>[4x]MSLTIGVIGKSVHPYWSQVEQGVKAAGKALGVDTKFFVPQKEDINAQLQMLESFIAEGVNGIAIA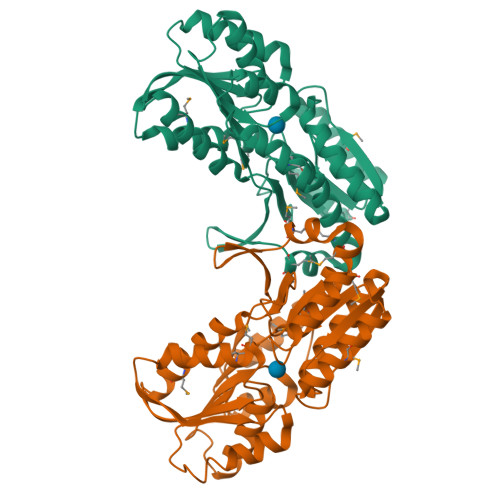PSDPTAVIPTIKKALEMGIPVVTLDTDSPDSGRYVYIGTDNYQAGYTAGLIMKELLGGKGKVVIGTGSLTAMNSLQRIQGFKDAIKDSEIEIVDILNDEEDGARAVSLAEAALNAHPDLDAFFGVYAYNGPAQALVVKNAGKVGKVKIVCFDTTPDILQYVKEGVIQATMGQRPYMMGYLSVTVLYLMNKIGVQNTLMMLPKVKVDGKVDYVIDTGVDVVTPENLDEYLKKMEELGIPIKEGHHHHHH GatD has sequence similarities to the catalytic domains of glutamine amidotransferases, while MurT is similar in sequence to the substrate-binding domains of Mur ligases. Together, these two proteins catalyze the amidation of α-D-isoglutamic acid of cell wall precursor stem peptides in an ATP-dependent reaction. In order to provide insight into the overall organization of this complex and to facilitate an understanding of the amidation mechanism, we have determined the crystal structure of the GatD/MurT complex. We find that the two proteins assemble into a curved, boomerang-shaped structure, with GatD docking to the C-terminal domain of MurT.

To obtain insight into interactions of the GatD/MurT complex with ATP, we prepared a ternary complex by soaking crystals with 2.1 mM of AMPPNP, an ATP analog. The structure of this complex was solved at 2.14 Å resolution using molecular replacement, and the corresponding electron density allowed us to unambiguously model AMPPNP into a binding site in the middle domain of MurT. The binding site contains the consensus sequence GTNGKT19, with residues K59 stabilizing the β and γ phosphate groups of AMPPNP and T60 coordinating a magnesium ion that is also contacted by the side chain of the conserved MurT-E108 residue. The magnesium ion helps in positioning the AMPPNP β and γ phosphates from the opposite side. The ATP molecule required for catalysis, replaced here by the non-hydrolyzable analog β,γ-imidoadenosine 5′-triphosphate (AMPPNP), is bound at the base of helix αm1 with the adenine moiety bound in a cleft formed next to helix αm1 while the phosphates are contacted by residues from strands βm1 and βm3. The observed binding mode is in excellent agreement with our mutagenesis data, as single or double mutants of nucleotide-binding site residues (T60A, E108A and N267Y) have completely lost their enzymatic activity. Complex formation with an ATP analog revealed a nucleotide-binding site in MurT that is similar to those found in other Mur ligases.

>[2x]MHELTIYHFMSDKLNLYSDIGNIIALRQRAKKRNIKVNVVEINETEGITFDECDIFFIGGGSDREQALATKELSKIKTPLKEAIEDGMPGLTICGGYQFLGKKYITPDGTELEGLGILDFYTESKTNRLTGDIVIESDTFGTIVGFENHGGRTYHDFGTLGHVTFGYGNNDEDKKEGIHYKNLLGTYLHGPILPKNYEITDYLLEKACERKGIPFEPKEIDNEAEIQAKQVLIDRANRQKKSRLEHHHHHH;>MRQWTAIHLAKLARKASRAVGKRGTDLPGQIARKVDTDVLRKLAEQVDDIVFISGTNGKTTTSNLIGHTLKANNIQIIHNNEGANMAAGITSAFIMQSTPKTKIAVIEIDEGSIPRVLKEVTPSMMVFTNFFRDQMDRFGEIDIMVNNIAETISNKGIKLLLNADDPFVSRLKIASDTIVYYGMKAHAHEFEQSTMNESRYCPNCGRLLQYDYIHYNQIGHYHCQCGFKREQAKYEISSFDVAPFLYLNINDEKYDMKIAGDFNAYNALAAYTVLRELGLNEQTIKNGFETYTSDNGRMQYFKKERKEAMINLAKNPAGMNASLSVGEQLEGEKVYVISLNDNAADGRDTSWIYDADFEKLSKQQIEAIIVTGTRAEELQLRLKLAEVEVPIIVERDIYKATAKTMDYKGFTVAIPNYTSLAPMLEQLNRSFEGGQS[2x]> YCTLSSGFTTVDISMAVGRVVVRPSDPVGKILRKATF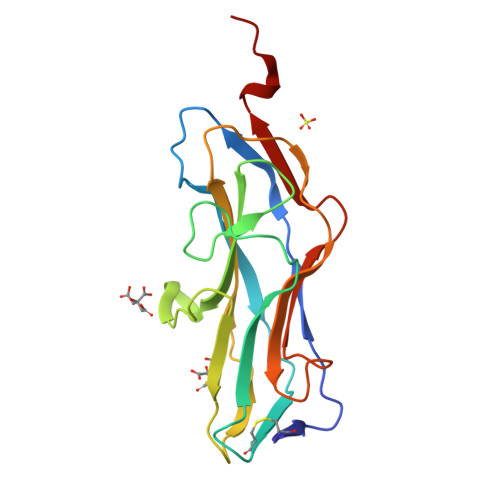PINPNGSTLRCTSYSDTITAALTQNYPLSPLGNSIYSTNIPGIGIRLYREAENATNFSGYYPYTRSLTPGTTYNLAQGYFVVEIVKTADQTGSGTLVPGLYSRYYVNGHMDRPFLTSTVYGNAITIASSSHHHHHH> MASWSHPQFEKGSMRDIVDPVFSIGISSLWDELRHMPAGGVWWFNVDRHEDAISLANQTIASQAETAHVAVISMDSDPAKIFQLDDSQGPE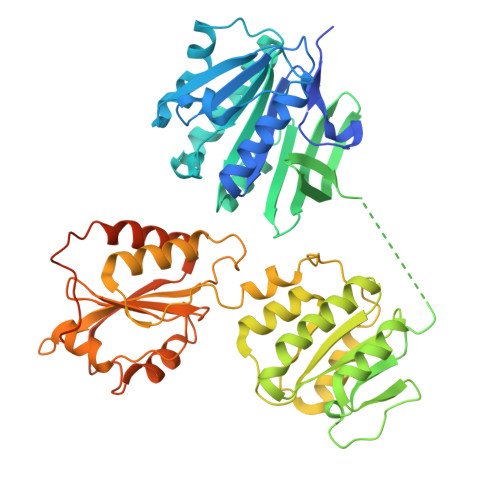KIKLFSMLNHEKGLYYLTRDLQCSIDPHNYLFILVCANNAWQNIPAERLRSWLDKMNKWSRLNHCSLLVINPGNNNDKQFSLLLEEYRSLFGLASLRFQGDQHLLDIAFWCNEKGVSARQQLSVQQQNGIWTLVQSEEAEIQPRSDEKRILSNVAVLEGAPPLSEHWQLFNNNEVLFNEARTAQAATVVFSLQQNAQIEPLARSIHTLRRQRGSAMKILVRENTASLRATDERLLLACGANMVIPWNAPLSRCLTMIESVQGQKFSRYVPEDITTLLSMTQPLKLRGFQKWDVFCNAVNNMMNNPLLPAHGKGVLVALRPVPGIRVEQALTLCRPNRTGDIMTIGGNRLVLFLSFCRINDLDTALNHIFPLPTGDIFSNRMVWFEDDQISAELVQMRLLAPEQWGMPLPLTQSSKPVINAEHDGRHWRRIPEPMRLLDDAVERSS~{N}2-methyl-~{N}4-[(1~{S},2~{S})-2-methylcyclopropyl]-6-[(~{S})-oxidanyl(phenyl)methyl]pyridine-2,4-dicarboxamide 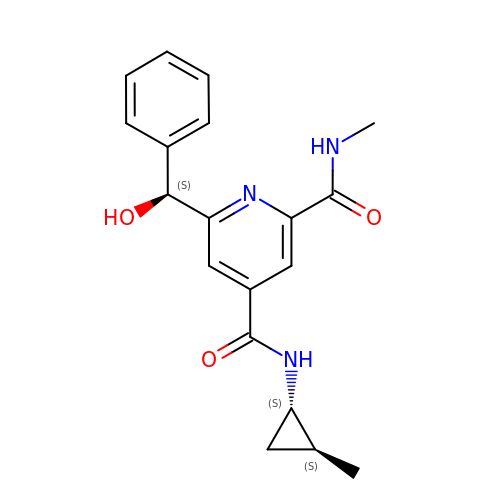| C19 H21 N3 O3 | OJSKWCXPUVTNCF-YLVFBTJISA-N>[2x]RDQSTPIIEVEGPLLSDTHVTFKLTMPSPMPEYLNVHYICESASRLLFLSMHWARSIPAFQALGQDCNTSLVRACWNELFTLGLAQCAQVMSLSTILAAIVNHLQN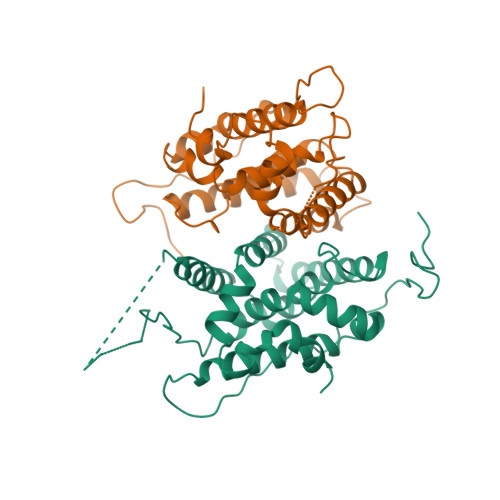SIQEDKLSGDRIKQVMEHIWKLQEFCNSMAKLDIDGYEYAYLKAIVLFSPDHPGLTSTSQIEKFQEAAQMELQDYVQATYSEDTYRLARILVRLPALRLMSSNITEELFFTGLIGNVSIDSIIPYILKMETAEYNGQITGASL>[4x]DKAT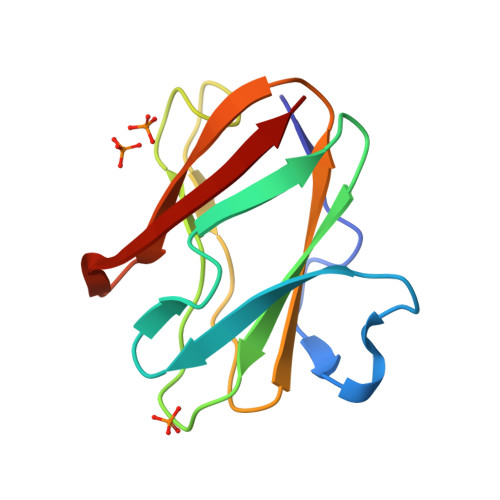IPSESPFAAAEVADGAIVVDIAKMKYETPELHVKVGDTVTWINREAMPHNVHFVAGVLGEAALKGPMMKKEQAYSLTFTEAGTYDYHCTPHPFMRGKVVVE>[12x]HHHHHHKIPNNPGAGENALEPIYIKDDDGYDIDTFLIPDHYKNYITKVLIPNGVLKNRIEKLAFDIKQVYRNEEFHVICLLKGSRGFFSALLKYLNRIHNYSSTESPKHLYVEHYVR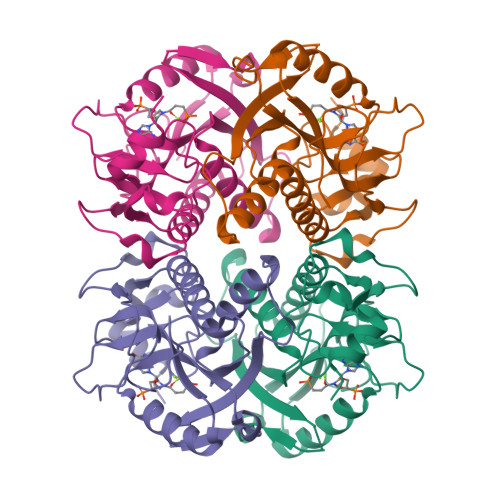VKSYCNDQSLDRIEIVSEDLSCLKDKHVLIVEDIIDTGKTLLKFCEYLKKFEVKTIAITCLFIKRTPLWNGFKADFVGFSIPDAFVVGYSLDYNEKFRDLDHLCLVNDEGIKKFRTAPPTA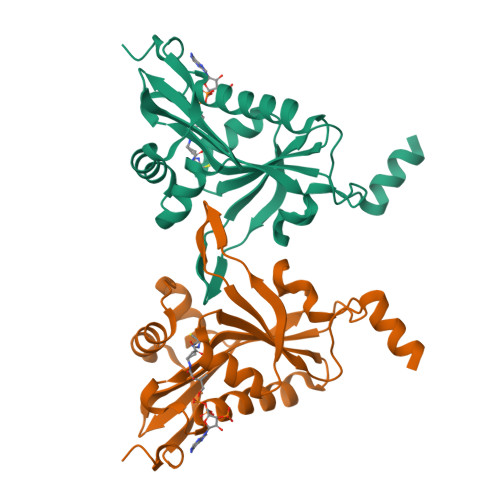> SMTEEERSSALSEVSLRLLCHDDIDTVKHLCGDWFPIEYPDSWYRDITSNKKFFSLAATYRGAIVGMIVAEIKNRTKIHKEDGDILASNFSVDTQVAYILSLGVVKEFRKHGIGSLLLESLKDHISTTAQDHCKAIYLHVLTTNNTAINFYENRDFKQHHYLPYYYSIRGVLKDGFTYVLYINGGHPPWTILDYIQHLGS>MRGSHHHHHHGSMDAQSAAKCLTAVRRHSPLVHSITNNVVTNFTANGLLALGASPVMAYAKEEVADMAKIAGALVLNIGTLSKESVEAMIIAGKSANEHGVPVILDPVGAGATPFRTESARDIIREVRLAAIRGNAAEIAHTVGVTDWLIKG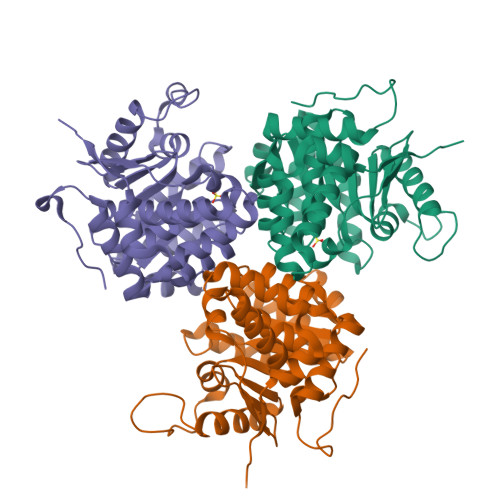VDAGEGGGDIIRLAQQAAQKLNTVIAITGEVDVIADTSHVYTLHNGHKLLTKVTGAGSLLTSVVGAFCAVEENPLFAAIAAISSYGVAAQLAAQQTADKGPGSFQIELLNKLSTVTEQDVQEWATIERVTVS[3x]> MHHHHHHHHHHGENLYFQGSDNIISFDHVTFTYPDSPRPALSDLSFAIERGSWTALIGHNGSGKSTVSKLINGLLAPDDLDKSSITVDGVKLGADTVWEVREKVGIVFQNPDNQFVGATVSDDVAFGLENRAVPRPEMLKIVAQAVADVGMADYADSEPSNLSGGQKQRVAIAGILAVKPQVIILDESTSMLDPEGKEQILDLVRKI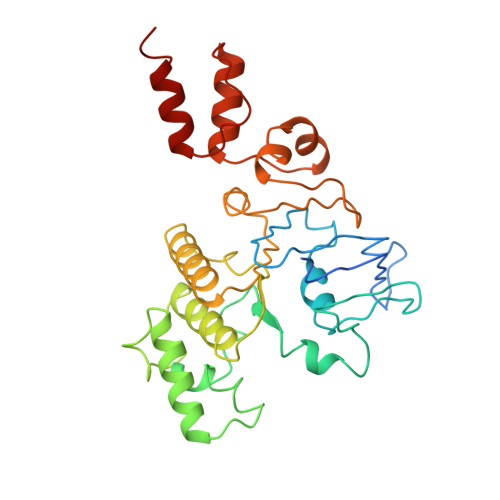KEDNNLTVISITHDLEEAAGADQVLVLDDGQLLDQGKPEEIFPKVEMLKRIGLDIPFVYRLKQLLKERGIVLPDEIDDDEKLVQSLWQLNSKM> ETNEITIGITVTTTGPAAALGIPERNALEFVAKEIGGHPLKVIVLDDGGDPTAATTNARRFVTESKADVIMGSSVTPPTVAVSNVANEAQVPHIALAPLPITPERAKWSVAMPQPIPIMGKVLYEHMKKNNIKTVGYIGYSDSYGDLWFNDLKKQGEAMGLKIVAEERFARPDTSVAGQVL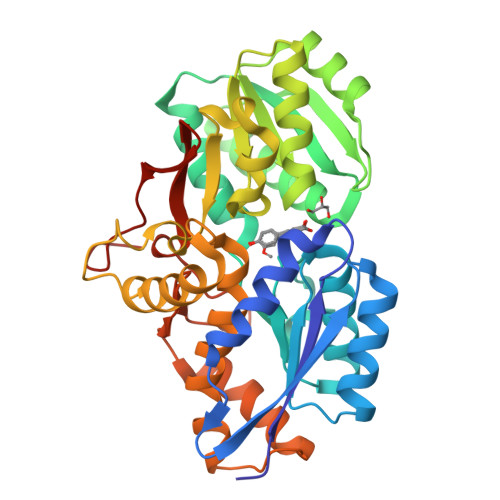KLVAANPDAILVGASGTAAALPQTSLRERGYKGLIYQTHGAASMDFIRIAGKSAEGVLMASGPVMDPEGQDDSALTKKPGLELNTAYEAKYGPNSRSQFAAHSFDAFKVLERVVPVALKTAKPGTQEFREAIRKALVSEKDIAASQGVYSFTETDRYGLDDRSRILLTVKDGKYVMVKAAALEHHHHHH>[4x]ILEAAVTQSPRNKVAVTGEKVTLSCQQTNNHNNMYWYRQDTGHGLRLIHYSYGAGSTEKGDIPDGYKASRPSQEQFSLILESATPSQTSVYFCASGGGGTLYFGAGTRLSVL;>ESQPDPMPDDLHKSSEFTGTMGNMKYLYDDHYVSATKVKSVDKFLAHDLIYNISDKKLKNYDKVKTELLNEDLAKKYKDEVVDVYGSNYYVNCYFSSKDGKVTGG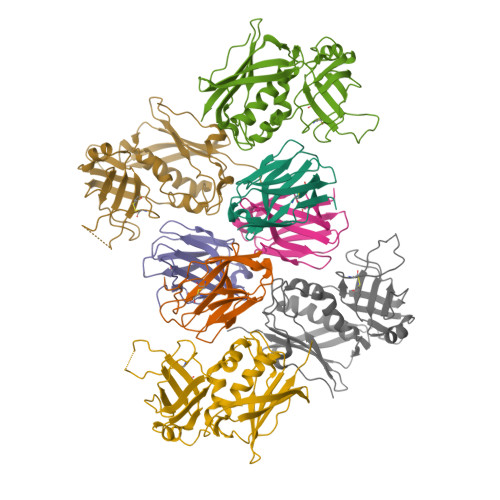KTCMYGGITKHEGNHFDNGNLQNVLVRVYENKRNTISFEVQTDKKSVTAQELDIKARNFLINKKNLYEFNSSPYETGYIKFIENNGNTFWYDMMPAPGDKFDQSKYLMMYNDNKTVDSKSVKIEVHLTTKNG[4x]> MEPSSKKLTGRLMLAVGGAVLGSLQFGYNTGVINAPQKVIEEFYNQTWVHRYGESILPTTLTTLWSLSVAIFSVGGMIGSFSVGLFVNRFGRRNSMLMMNLLAFVSAVLMGFSKLGKSFEMLILGRFIIGVYCGLTTGFVPMYVGEVSPTALRGALGTLHQLGIVVGILIAQVFGLDSIMGNKDLWPLLLSIIFIPALLQCIVLPFCPESPRFLLINRNEENRAKSVLKKLRGTADVTHDLQEMKEESRQMMREKK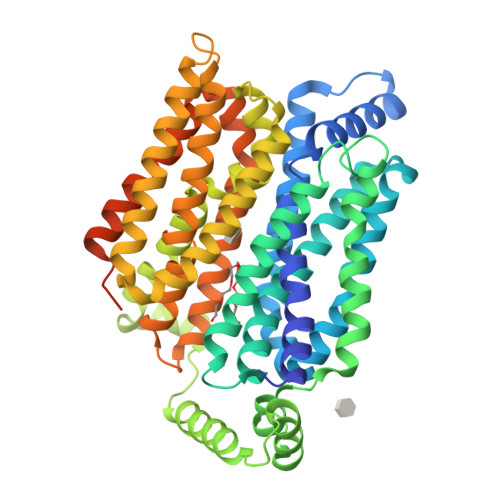VTILELFRSPAYRQPILIAVVLQLSQQLSGINAVFYYSTSIFEKAGVQQPVYATIGSGIVNTAFTVVSLFVVERAGRRTLHLIGLAGMAGCAILMTIALALLEQLPWMSYLSIVAIFGFVAFFEVGPGPIPWFIVAELFSQGPRPAAIAVAGFSNWTSNFIVGMCFQYVEQLCGPYVFIIFTVLLVLFFIFTYFKVPETKGRTFDEIASGFRQGGASQSDKTPEELFHPLGADSQVLVPR> HMLAADVPTGCVTIKNRHEGRYLAHSISTHDADRRHVSFCTDPQRWTITAEGTNFRIRNNKHGEELFESQQKFNGNYVFL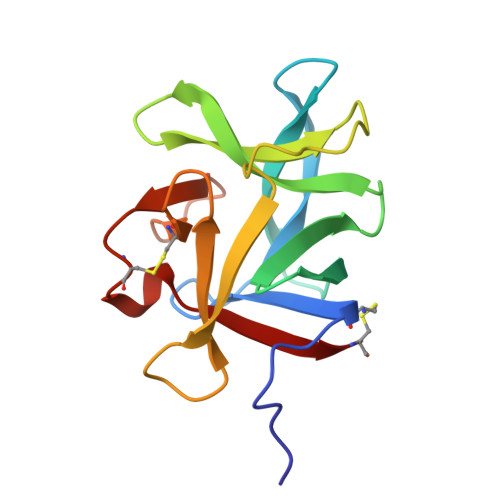WIKKSLINDGGASWKITESGNPGYFHIKNVKFSHCLFTQGGTDWVAAYESCDTAKYEWRIVKC In eukaryotes, the core Sec61 channel forms a larger translocon associating with the multimeric translocon-associated protein (TRAP) complex and oligosaccharyltransferase (OST) complexes. In the Sec61/OST/TRAP translocon, the TRAP complex aids ribosome docking to the Sec61 translocon and participates in protein folding, while the OST complex mediates N-linked glycosylation. Phylogenetic analyses indicate the inheritance of eukaryotic Sec61/oligosaccharyltransferase/translocon-associated protein translocon subunits from an Asgard archaea ancestor. Asgard archaea are predicted to have a complete Sec61αβγ complex and many of the components of the OST and TRAP complexes.

To probe the global structural similarities between the MK-D1 and eukaryotic Sec61/OST/TRAP translocons, we constructed the AF2 predicted models of MK-D1 Sec61, OST and TRAP complexes and superimposed them onto the eukaryotic Sec61/OST/TRAP translocon cryo-electron microscopy (cryoEM) structure. We were particularly intrigued by the cytoplasmic C-terminal domain of OST1, which forms a cytoplasmic helical bundle in the MK-D1 model and in the eukaryotic structure (circled). To confirm the validity of the AF2 model in this region, we expressed, purified, crystallized, and solved the X-ray structure of this domain. Finally, to ascertain whether this cytoplasmic domain of MK-D1 OST1 can interact with ribosomes, we produced histidine-tagged domains from MK-D1 and human OST1 and carried out pulldowns on nickel-nitrilotriacetic acid (NTA) beads against HeLa cell lysate, and semi-purified and highly purified human ribosomes. Ribosomes were detected to bind to the human and MK-D1 cytoplasmic C-terminal domains of OST1, but not to the negative control, the MK-D1 OST1 extracellular N-terminal domains. The C-terminal domains of OST1 were able to recruit ribosomes from samples with different levels of ribosome purity, indicating a direct and specific interaction. This finding suggests that MK-D1 OST1 participates in the recruitment of MK-D1 ribosomes to the Sec61/OST/TRAP translocon at the cell membrane for translation and translocation of membrane proteins and preproteins. A comparison of the surface residues of the human and MK-D1 cytoplasmic C-terminal domains of OST1 reveals surface patches of basic residues that cluster in regions that may be able to interact with the RNA components of the ribosome. Here, we show that the cytoplasmic C-terminal domain of archaea OST1 also mediates interactions with the ribosome, and specifically, the MK-D1 OST1 complex can engage human ribosomes, despite the ∼1.8 BY of divergence of the two species. Furthermore, we show that the cytoplasmic domain of Candidatus Prometheoarchaeum syntrophicum strain MK-D1 oligosaccharyltransferase 1 (ribophorin I) can interact with eukaryotic ribosomes.

> GPRKQRKDYEEGEESFIEQSVPIRELTRFVTLIEEKNAILLDIEKADSDLRRKRIQKKVYTKTVKNYQNKLKELNEESIPFKRILMETGGQIQSIIQKLDFLEAEKISVKDSVKLLKDRYKRGKLPSKAAYERLSSDMIKQLASSQNKIDRYINELRAYII>MRYAFPTQQLKDNVMQTVKLNNGIAMPLLGFGVFQMTNTAECERAVIDAIETGYRLIDTAASYQNETQVGNALKLSGIARDELFITTKLWLQDTYYEGAKAQFERSLNRLQLDYVDLYLIHQPYGDVHGAWRAMEELHQAGKIRAIGVSNFHPDRLADLMAFNKIIPAVNQIEVNPFNQQLHAVPWMQSRGIQPEAWAPFAEGRNGLFQNPVLTAIGEKYGKSVGQVVLRWIFQRGIVSLAKSVRKGRMEENINILDFELSAEDMLQIAALDTATSAFFSHRDPAMVEWLTGRKLD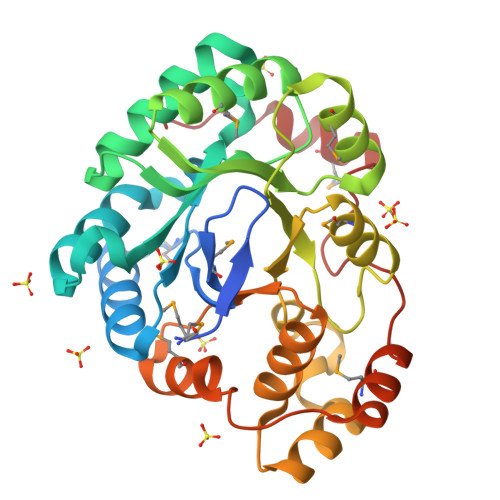V[6x]> ASITEIKADKTTAVANGQDAITYTVKVMKGDKPVSNQEVTFTTTLGKLSNSTEKTDTNGYAKVTLTSTTPGKSLVSAR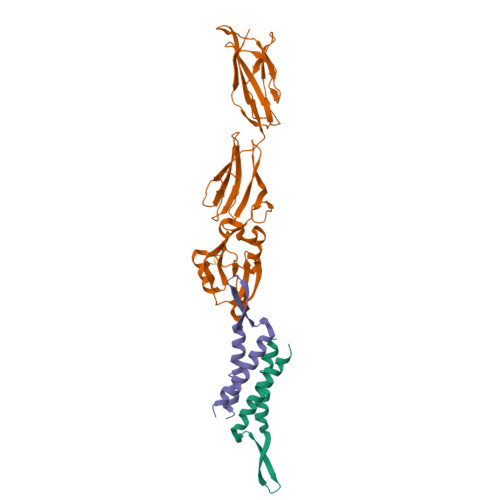VSDVAVDVKAPEVEFFTTLTIDDGNIEIVGTGVKGKLPTVWLQYGQVNLKASGGNGKYTWRSANPAIASVDASSGQVTLKEKGTTTISVISSDNQTATYTIATPNSLIVPNMSKRVTYNDAVNTCKNFGGKLPSSQNELENVFKAWGAANKYEYYKSSQTIISWVQQTAQDAKSGVASTYDLVKQNPLNNIKASESNAYATCVK;> MDQAANAAESATKDQLTQEAFKNPENQKVNIDANGNAIPSGELKDDIVEQIAQQAKEAGEVARQQA>[2x]MAQILPIRFQEHLQLQNLGINPANIGFSTLTMESDKFICIREKVGEQAQVVIIDMNDPSNPIRRPISADSAIM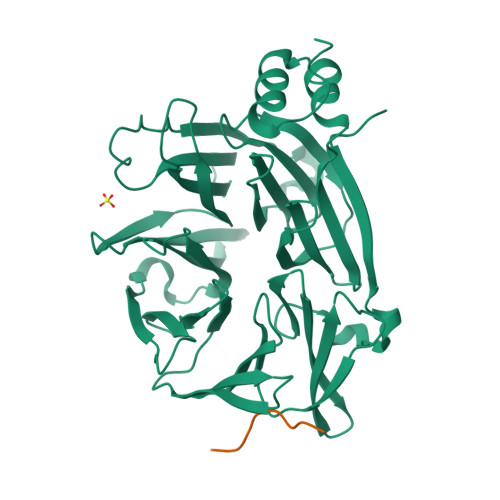NPASKVIALKAGKTLQIFNIEMKSKMKAHTMTDDVTFWKWISLNTVALVTDNAVYHWSMEGESQPVKMFDRHSSLAGCQIINYRTDAKQKWLLLTGISAQQNRVVGAMQLYSVDRKVSQPIEGHAASFAQFKMEGNAEESTLFCFAVRGQAGGKLHIIEVGTPPTGNQPFPKKAVDVFFPPEAQNDFPVAMQISEKHDVVFLITKYGYIHLYDLETGTCIYMNRISGETIFVTAPHEATAGIIGVNRKGQVLSVCVEEENIIPYITNVLQNPDLALRMAVRNNLAGAEELF;>[2x]SDHSVDLITFDSVTDIY1-{1-[8-(1-ethyl-5-methyl-1H-pyrazol-4-yl)-9-methyl-9H-purin-6-yl]piperidin-4-yl}-1,3-dihydro-2H-imidazo[4,5-b]pyridin-2-one | C23 H26 N10 O | 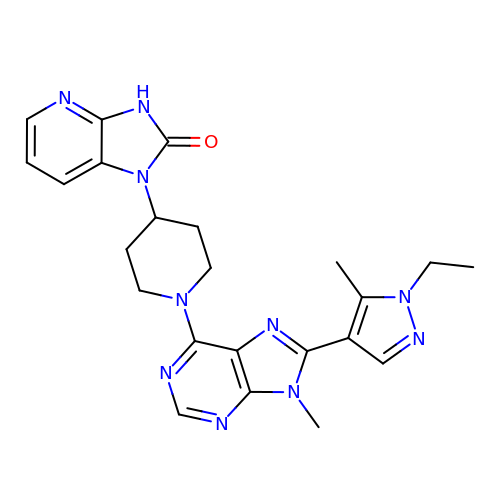WRPLWRLROFHFJF-UHFFFAOYSA-N In contrast to its eukaryotic counterparts, bacterial HSS synthesizes 1 mol HSP from 2 mol PUT. NAD+ serves as a non-covalently bound prosthetic group for BvHSS. The interface area of the dimer was calculated as approximately 1700 Å2 by PDBsum indicating a stable dimer23. The BvHSS subunit consists of two domains as determined by CATH24: one “NAD(P)-binding Rossmann-like” domain (domain 1, residues 3–163 and 394–425) and one “homospermidine-synthase-like domain” (domain 2, residues 164–395 and 426–477) as shown in Fig. 2a and S1. The crystal structures of BvHSS containing NAD+ clearly show that the active site is localized inside each subunit.

Based on these observations, four variants of BvHSS (N162D, E237Q, H296S, and E298Q) have been generated for further characterization of residues within the active site. Residue Glu-298 has been chosen based on direct interaction with the active site residue His-296, forming a Glu-His-Glu triad together with Glu-237. All four variants of BvHSS lead to enzymatically inactive but soluble enzymes. All BvHSS and BvHSS variants co-crystallized with AGM were found to have AGM bound to the protein surface at various sites, most likely causing the observed improvement in crystal growth. In contrast to wild-type BvHSS, the variant H296S was found to bind AGM within the active site. The guanidine group of AGM was approximately placed at the former His-296 imidazole ring position. The primary amino group of AGM was bound and coordinated as that of HSP or PUT at the inner amino site. The side chain of His-296 seems to be crucial for correct substrate positioning.

>DWPVYHRIDGPIVMIGFGSIGRGTLPLIERHFAFDRSKLVVIDPSDEARKLAEARGVRFIQQAVTRDNYRELLVPLLTAGPGQGFCVNLSVDTSSLDIMELARENGALYIDTVVEPWLGFYFDPDLKPEARSNYALRETVLAARRNKPGGTTAVSCCGANPGMVSWFVKQALVNLAADLGVTGEEPTTREEWARLAMDLGVKGIHIAERDTQRASFPKPFDVFVNTWSVEGFVSEGLQPAELGWGTFERWMPDNARGHDSGCGAGIYLLQPGANTRVRSWTPTAMAQYGFLVTSNESISIADFLTVRDAAGQAVYRPTCHYAYHPCNDAVLSLHEMFGSGKRQSDWRILDETEIVDGIDELGVLLYGHGKNAYWYGSQLSIEETRRIAPDQNATGLQVSSAVLAGMVWALENPNAGIVEADDLDFRRCLEVQTPYLGPVVGVYTDWTPLAGRPGLFPEDIDTSDPWQFRNVLVR[2x]Deoxyribozymes (DNAzymes) are short (15–40 nt) single-stranded DNA molecules that catalyze chemical reactions. DNAzymes generally consist of two substrate binding arms flanking a central catalytic core. The RNA-cleaving 10-23 DNAzyme was the first DNAzyme to be evolved and possesses clinical and biotechnical applications as a biosensor and a knockdown agent. Despite this, a lack of structural and mechanistic information has hindered the optimization and application of the 10-23 DNAzyme.

To address this need, we have obtained a 2.7 Å crystal structure of the 10-23 DNAzyme-substrate complex captured in precatalytic conditions. To combat the crystallization forces contributing to artifact formation, the substrate and DNAzyme were placed on the same continuous ssDNA strand with a snapback GAAA tetraloop to allow for alignment of the scissile phosphate within the DNAzyme catalytic core. This oligonucleotide contains a single ribonucleotide position (−1A), that uses its 2′-OH as the attacking nucleophile to cleave the adjacent 3′ phosphoribose backbone position. To capture a precatalytic 10-23 DNAzyme structure, the 2′-OH position of the RNA nucleophile was modified by 2′-O-methyl (2′-OMe) substitution which was shown to attenuate activity in vitro. The structure exhibits a homodimer conformation with extensive base pairing occurring throughout the 10-23 DNAzyme catalytic core. The dimer is mediated through two regions of antiparallel base pairing within the catalytic core. The region (G2-C7) is palindromic and is responsible for most of the base pair interactions that occur within the dimer. In this structure of the 10-23 DNAzyme, a bend is observed at the scissile phosphate and is coordinated through base pair interaction with the substrate binding arms at the −1 and +1 positions relative to the catalytic core and with G1 forming a non-canonical G-A base pair with the ribo-adenosine at the cleavage site. The captured precatalytic active site conformation does not align the 2′-OH nucleophile with the scissile phosphate in the pre-requisite in-line attack conformation often observed in RNA-cleaving machines. Two magnesium ions are observed to coordinate to the 2′-OH nucleophile, 3′ bridging oxygen, and the 5′ leaving group of the cleavage site.

>[2x]SMLTLIQGKKIVNHLRSRLAFEYNGQLIKILSKNIVAVGSLRREEKMLNDVDLLIIVPEKKLLKHVLPNIRIKGLSFSVKVCGERKCVLFIEWEKKTYQLDLFTALAEEKPYAIFHFTGPVSYLIRIRAALKKKNYKLNQYGLFKNQTLVPLKITTEKELIKELGFTYRIPKKRL>MTRLSEILDQMTTVLNDLKTVMDAEQQQLSVGQINGSQLQRITEEKSSLLATLDYLEQQRRLEQNAQRSANDDIAERWQAITEKTQHLRDLNQHNGW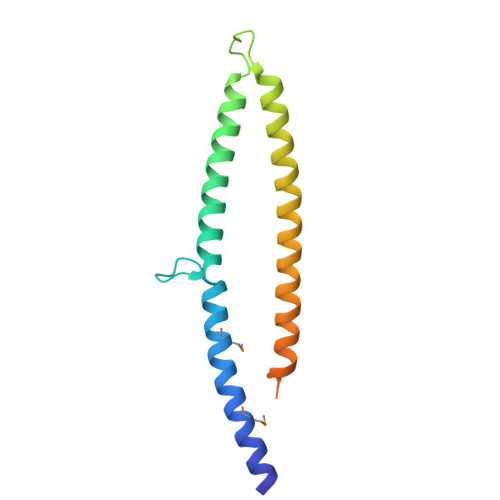LLEGQIERNQQALEVLKPHQEPTLYGADGQTSVSHRGGKKISI[4x]> GPLGSPEFPGRLEMEPDFYCVKWIPWKGEQTPIITQSTNGPCPLLAIMNILFLQWKVKLPPQKEVITSDELMAHLGNCLLSIKPQEKSEGLQLNFQQNVDDAMTVLPKLATGLDVNVRFTGVSDFE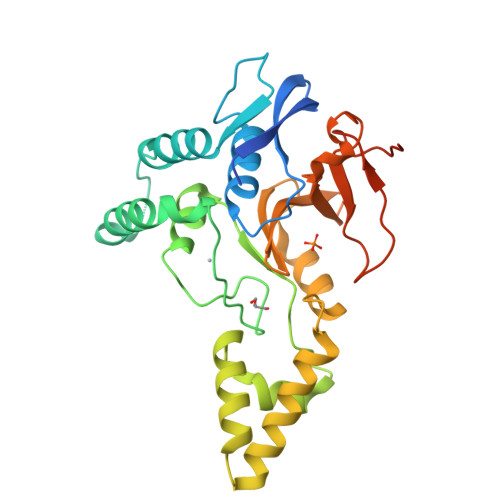YTPECSVFDLLGIPLYHGWLVDPQSPEAVRAVGKLSYNQLVERIITCKHSSDTNLVTEGLIAEQFLETTAAQLTYHGLCELTAAAKEGELSVFFRNNHFSTMTKHKSHLYLLVTDQGFLQEEQVVWESLHNVDGDSCFCDSDFHLSHSLGKGPGAEGGSGSPE4-amino-N-methyl-2-[4-(morpholin-4-yl)phenyl]thieno[3,2-c]pyridine-7-carboxamide 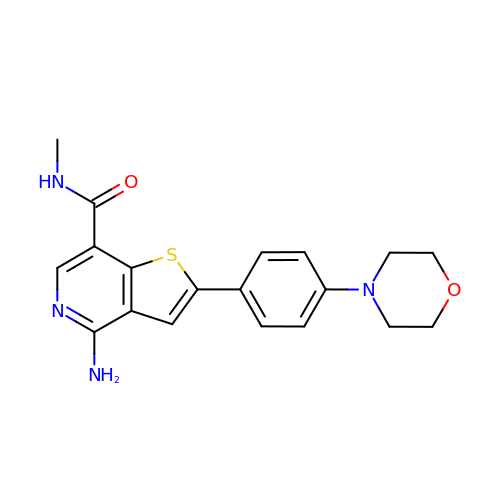| C19 H20 N4 O2 S | JNNQSTULXLHQBB-UHFFFAOYSA-N>[3x]SKKPSLSVQPGPVMAPGES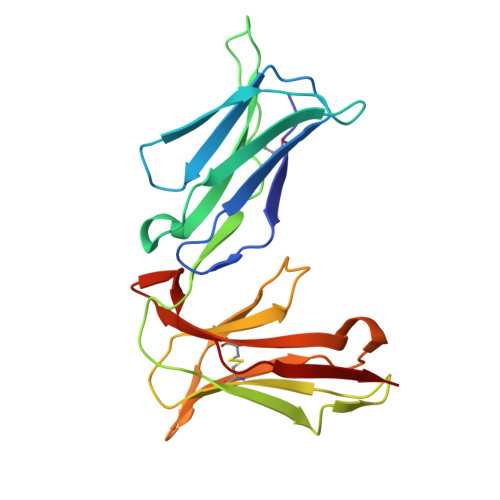LTLQCVSDVGYDRFVLYKEGERDLRQLPGRQPQAGLSQANFTLGPVSRSYGGQYRCYGAHNLSSECSAPSDPLDILITGQIRGTPFISVQPGPTVASGENVTLLCQSWRQFHTFLLTKAGAADAPLRLRSIHEYPKYQAEFPMSPVTSAHAGTYRCYGSLNSDPYLLSHPSEPLELVVS> MYVLFVCLIDSMNVEEGKQIKEMILPHNNRQLARQYFDSLPENDINRKYYEGLKYETPKTFFGRFLNQFNIDAKLDTLSKFYTYQKTIRATQAELQEDRKSYLTNSLLFTAVSWFSIYQFARKGAVLPVLREYGRYFGTHRLFRQYLHTLVLPLLYTEYALNQKYYTHMEHLWTVHVNRLNQKILEDPLYTFYPQELNVPKHNIIVPTIFRDTP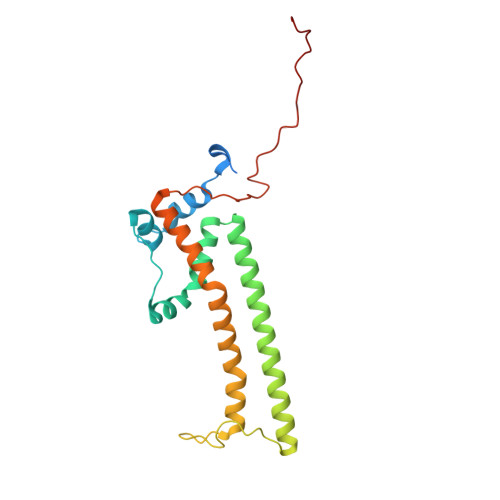Q> ADNLAEFHVQNQECDSCHTPDGELSNDSLTYENTQCVSCHGTLAEVAETTKHEHYNAHASMFPGEVACTSCHSAHEKSMVYCDSCHSFDFNMPYAKKWLRDEPTIAELAKDKSERQAALASAPHDTVDVVVVGSGGAGFSAAISATDSGAKVILIEKEPVIGGNAKLAAGGMNAAWTDQQKAKKITDSPELMFEDTMKGGQNINDPALVKVLSSHSKDSVDWMTAMGADLTDVGMMGGASVNRAHRPTGGAGVGAHVVQVLYDNAVKRNIDLRMNTRGIEVLKDDKGTVKGILVKGMYKGYYWVKADAVILATGGFAKNNERVAKLDPSLKGFISTNQPGAVGDGLDVAE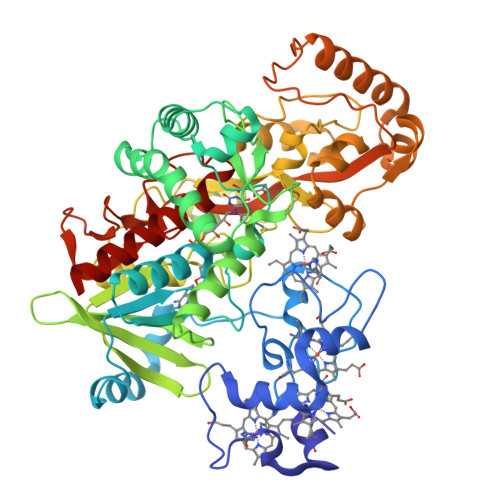NAGGALKDMQYIQAHPTLSVKGGVMVTEAVRGNGAILVNREGKRFVNEITTRDKASAAILAQTGKSAYLIFDDSVRKSLSKIDKYIGLGVAPTADSLVKLGKMEGIDGKALTETVARYNSLVSSGKDTDFERPNLPRALNEGNYYAIEVTPGVHHTMGGVMIDTKAEVMNAKKQVIPGLYGAGEVTGGVHGANRLGGNAISDIITFGRLAGEEAAKYSKKN> MGHHHHHHRKVQMGAKDATPVPCGRWAKILEKDKRTQQMRMQRLKAKLQMPFQSGEFKALTRRLQVEPRLLSKQMAGCLEDCTRQAPESPWEEQLARLLQEAPGKLSLDVEQAPSGQHSQAQLSGQQQRLLAFFKCCLLTDQLPLAHHLLVVHHGQRQKRKLLTLDMYNAVMLGWARQGAFKELVYVLFMVKDAGLTPDLLSYAAALQCMGRQDQDAGTIERCLEQMSQEGLKLQALFTAVLLSEEDRATVLKAVHKVKPTFS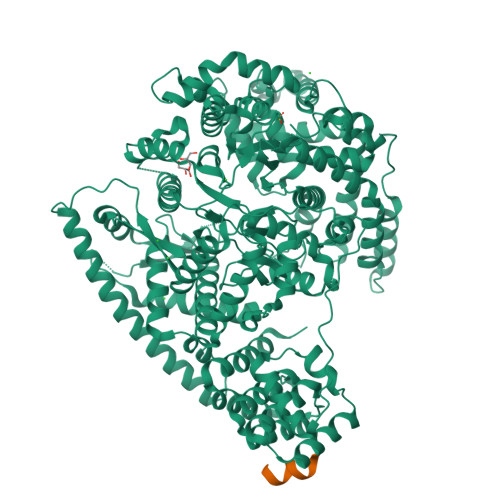LPPQLPPPVNTSKLLRDVYAKDGRVSYPKLHLPLKTLQCLFEKQLHMELASRVCVVSVEKPTLPSKEVKHARKTLKTLRDQWEKALCRALRETKNRLEREVYEGRFSLYPFLCLLDEREVVRMLLQVLQALPAQGESFTTLARELSARTFSRHVVQRQRVSGQVQALQNHYRKYLCLLASDAEVPEPCLPRQYWEALGAPEALREQPWPLPVQMELGKLLAEMLVQATQMPCSLDKPHRSSRLVPVLYHVYSFRNVQQIGILKPHPAYVQLLEKAAEPTLTFEAVDVPMLCPPLPWTSPHSGAFLLSPTKLMRTVEGATQHQELLETCPPTALHGALDALTQLGNCAWRVNGRVLDLVLQLFQAKGCPQLGVPAPPSEAPQPPEAHLPHSAAPARKAELRRELAHCQKVAREMHSLRAEALYRLSLAQHLRDRVFWLPHNMDFRGRTYPCPPHFNHLGSDVARALLEFAQGRPLGPHGLDWLKIHLVNLTGLKKREPLRKRLAFAEEVMDDILDSADQPLTGRKWWMGAEEPWQTLACCMEVANAVRASDPAAYVSHLPVHQDGSCNGLQHYAALGRDSVGAASVNLEPSDVPQDVYSGVAAQVEVFRRQDAQRGMRVAQVLEGFITRKVVKQTVMTVVYGVTRYGGRLQIEKRLRELSDFPQEFVWEASHYLVRQVFKSLQEMFSGTRAIQHWLTESARLISHMGSVVEWVTPLGVPVIQPYRLDSKVKQIGGGIQSITYTHNGDISRKPNTRKQKNGFPPNFIHSLDSSHMMLTALHCYRKGLTFVSVHDCYWTHAADVSVMNQVCREQFVRLHSEPILQDLSRFLVKRFCSEPQKILEASQLKETLQAVPKPGAFDLEQVKRSTYFFS FdlA from Flavobacterium sp. SA-0082 is an endo-type fucoidan-degrading enzyme that cleaves the sulfated fuco-glucuronomannan (SFGM) through a lytic mechanism. We show that the FdlA-NTD adopts a right-handed parallel β-helix fold, and possesses a substrate binding site composed of a long groove and a unique alkaline pocket. Our structural, biochemical, and enzymological analyses strongly suggest that FdlA-NTD utilizes catalytic residues different from other β-helix polysaccharide lyases, potentially representing a novel polysaccharide lyase family. Here, we report crystal structures and enzymological characterization of wild type (WT) and eight single mutants of the catalytic N-terminal domain (NTD) of FdlA, revealing its unique substrate binding pocket and identifying the key catalytic residues.

We solved the crystal structure of FdlA-NTD WT at 1.3 Å resolution using the single-wavelength anomalous diffraction (SAD) method. In the FdlA-NTD structure, two molecules are present in an asymmetric unit and adopt nearly identical conformations, with a root-mean-squares deviation (RMSD) of 0.11 Å for all Cα atoms. FdlA-NTD forms a right-handed parallel β-helix, one type of the six PL classes, shaping like a fish skeleton with a dimension of 67 Å × 22 Å × 47 Å. The FdlA-NTD molecule contains 13 coils, with coils 1–6 being complete, while the other coils lacking either PB1 or PB3. The T3 loops at coils 1–9 together with the adjacent PB1 sheets form a 30-Å long concave groove at the surface of the β-helix. In contrast to other PL enzymes, which form a planar groove, FdlA-NTD extends its C-terminal part of the surficial groove into a deep pocket, measuring 11 Å × 13 Å × 8 Å. The region comprising the deep pocket and the C-terminal part of the groove (between coil 5 and coil 9) is characterized by a strong positive charge, which is unfavorable for metal binding due to the electrostatic repulsion. Moreover, we observed several bulbs of non-protein densities in the ‘groove-pocket’ region, and modeled these densities as three sulfate groups (S1–S3), based on the density shape and the fact that high concentration of sulfate ammonium was added in the crystallization reagent. One sulfate S1 is located in the alkaline pocket, strongly indicating that the positively charged pocket facilitates the attraction and interaction with the negative charged sulfate groups of fucoidans, explaining the previous observation that FdlA can only cleave fucoidans containing sulfated fucoses. In addition to these common stacks and ladders, we also found an unusual cysteine ladder composed of five cysteine residues (Cys168, Cys192, Cys267, Cys290, Cys309) that are located at the T2-PB3 juncture of coils 4–8, beneath the potential substrate binding groove.

>[2x]HHHHHHSSGLVPRGSHMQTTTVYSLEDLLPYLKQDNVDVKLAPGTYNVNGFDVGEDRLFSTTPLFLFEGSNSTYDFTDVKLNINTVVLTKFGNNEVNEIQILGNNNVLKNLKLEDIGTTAPSNRAQSIVIDGRDNRIEGFHLTIRGSYPYGYGDAFGKGGGSVINHRKHSGVLIRGLRNHLKDCTIISRSYGHIVFMQAASYPTVEGCYIEGEMRSTDDMLAEEGTGSPADKVDFMTVWGYKLPAGYMMSLQEGGIRAYNAGTTYIDGVEIQRATDNPTVLNCTIKNARTGVTLAHANGTKYVEGCTVLGCENGYSIGSGTVVNCGADAIYGPVFKNTYGSDKGYNADITILPPSDAYYNGHDAVAYIGGSNHNLTFRSEITEIPSNLKIMVSGDLQGLRVLHGSNPSQNNFAGTNIVLRNLTNFPVDLHSDSSNITVTSCDTDNITDNGTNNSIEAIDCDSD> SPILGYWKIKGLVQPTRLLLEYLEEKYEEHLYERDEGDKWRNKKFELGLEFPNLPYYIDGDVKLTQSMAIIRYIADKHNMLGGCPKERAEISMLEGAVLDIRYGVSRIAYSKDFETLKVDFLSKLPEMLKMFEDRLCHKTYLNGDHVTHPDFMLYDALD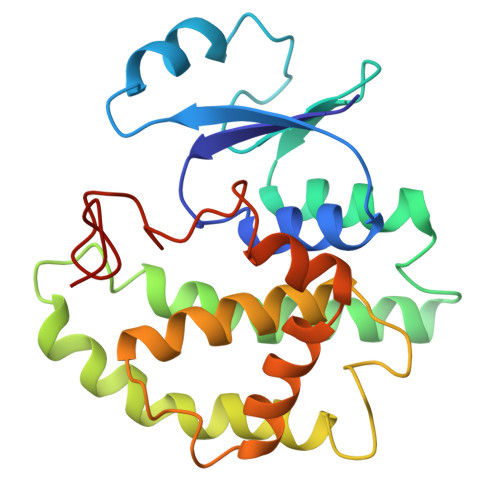VVLYMDPMCLDAFPKLVCFKKRIEAIPQIDKYLKSSKYIAWPLQGWQATFGGGDHPPKSD>[8x]MLKGKKAVVTGST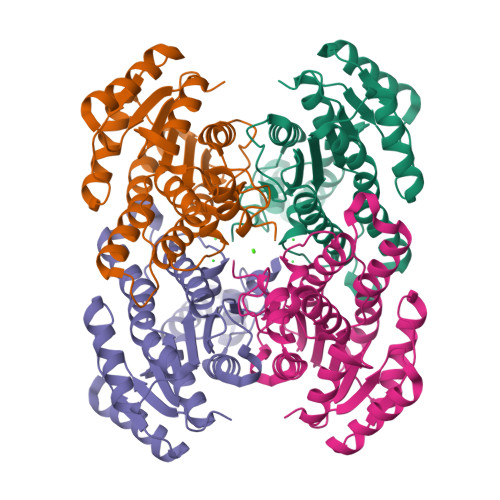SGIGLAMATELAKAGADVVINGFGQPEDIERERSTLESKFGVKAYYLNADLSDAQATRDFIAKAAEALGGLDILVNNAGIQHTAPIEEFPVDKWNAIIALNLSAVFHGTAAALPIMQKQGWGRIINIASAHGLVASVNKSAYVAAKHGVVGLTKVTALENAGKGITCNAICPGWVRTPLVEKQIEAISQQKGIDIEAAARELLAEKQPSLQFVTPEQLGGAAVFLSSAAADQMTGTTLSLDGGWTAR>MFENITAAPADPILGLADLFRADERPGKINLGIGVYKDETGKTPVLTSVKKAEQYLLENETTKNYLGIDGIPEFGRCTQELLFGKGSALINDKRARTAQTPGGTGALRVAADFLAKNTSVKRVWVSNPSWPNHKSVFNSAGLEVREYAYYDAENHTLDFDALINSLNEAQAGDVVLFHGCCHNPTGIDPTLEQWQTLAQLSVEKGWLPLFDFAYQGFARGLEEDAEGLRAFAAMHKELIVASSYSHNFGLYNERVGACTLVAADSETVDRAFSQMKAAIRANYSNPPAHGASVVATILSNDALRAIWEQELTDMRQRIQRMRQLFVNTLQE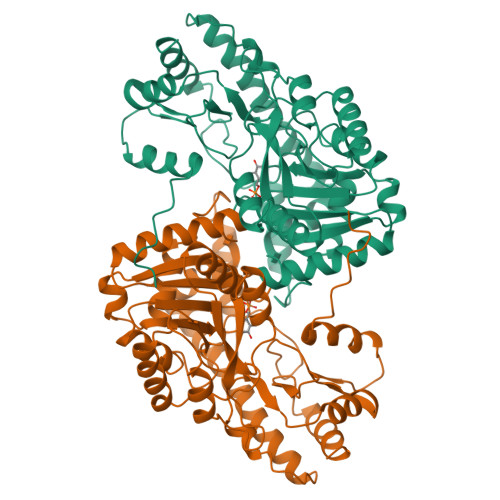KGANRDFSFIIKQNGMFSFSGLTKEQVLRLREEFGVYAVASGRVNVAGMTPDNMAPLCEAIVAVL[2x]> 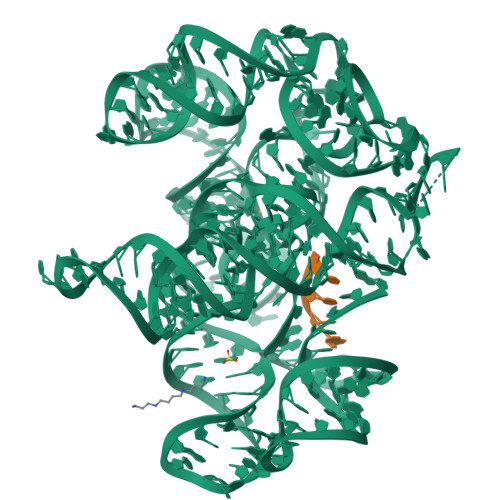GAGCCUUUAUACAGUAAUGUAUAUCGAAAAAUCCUCUAAUUCAGGGAACACCUAAGGCAAUCCUGAGCUAAGCUCUUAGUAAUAAGAGAAAGUGCAACGACUAUUCCGAUAGGAAGUAGGGUCAAGUGACUCGAAAUGGGGAUUACCCUUCUAGGGUAGUGAUAUAGUCUGAACAUAUAUGGAAACAUAUAGAAGGAUAGGAGUAACGAACCUAUCCGUAACAUAAUUG;> GCUU> QKDANFASGRNSIVHLFEWKWNDIADECERFLQPQGFGGVQISPPNEYLVADGRPWWERYQPVSYI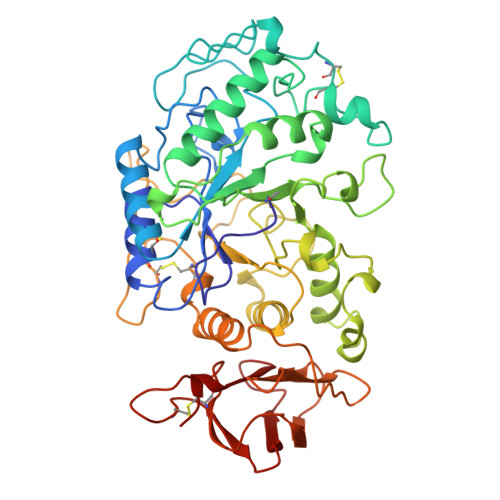INTRSGDESAFTDMTRRCNDAGVRIYVDAVINHMTGMNGVGTSGSSADHDGMNYPAVPYGSGDFHSPCEVNNYQDADNVRNCELVGLRDLNQGSDYVRGVLIDYMNHMIDLGVAGFRVDAAKHMSPGDLSVIFSGLKNLNTDYGFADGARPFIYQEVIDLGGEAISKNEYTGFGCVLEFQFGVSLGNAFQGGNQLKNLANWGPEWGLLEGLDAVVFVDNHDNQRTGGSQILTYKNPKPYKMAIAFMLAHPYGTTRIMSSFDFTDNDQGPPQDGSGNLISPGINDDNTCSNGYVCEHRWRQVYGMVGFRNAVEGTQVENWWSNDDNQIAFSRGSQGFVAFTNGGDLNQNLNTGLPAGTYCDVISGELSGGSCTGKSVTVGDNGSADISLGSAEDDGVLAIHVNAKL> TAVVTN

Transthyretin (TTR)3 is a 55-kDa protein that aggregates into amyloid fibrils under pathological conditions. In its native tetrameric conformation, TTR transports retinol-binding protein and thyroxine (T4) in the blood and cerebrospinal fluid. Amyloid aggregation of TTR occurs by dissociation of tetrameric TTR into monomers; these partially unfold into amyloidogenic intermediates and self-associate into soluble oligomers and amyloid aggregates. Here we identify two segments of TTR that drive protein aggregation by self-association and formation of steric zipper spines of amyloid fibrils.

Next, we performed structural analysis of the isolated strand H segment to test whether it forms a steric zipper structure. We found that 119TAVVTN124 forms a Class-2 steric zipper (Ref. 25 and Fig. 3D) in which the β-strands stack into parallel β-sheets with one sheet face packing against another sheet back. The side chain organization explains why the residue replacements E92P and V94P hinder TTR aggregation because the proline substitution would decrease the shape complementarity between sheets in the steric zipper structure. Moreover, the crystal structure of 119TAVVTN124 is a Class-2 steric zipper, face-to-back arrangement with parallel β-strands and parallel sheets (Ref. 25 and Fig. 3D). The side chain organization in this peptide also explains why the residue replacements T119W, T119Y, V121W, and V121Y impede TTR aggregation. Taken together, these experiments suggest that the 119TAVVTN124 segment is important for fibril formation. For additional evidence, we synthesized and analyzed 6-residue peptides containing the same substitutions, and they did not form aggregates or fibrils in isolation. First, peptides with Tyr/Trp substitutions did not form fibrils in isolation.N7-(3,4-difluorobenzyl) guanine 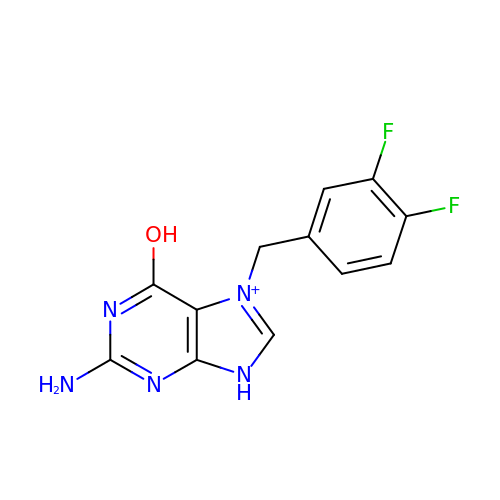| C12 H10 F2 N5 O | NBTRICCNNMIXFE-UHFFFAOYSA-O>[10x]MVTTVLWGCELSQERRTWTFRPQLEGKQSCR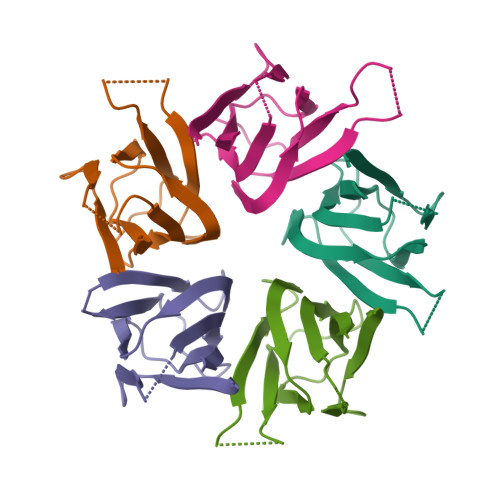LLLHTICLGEKAKEEMHRVEILPPANQEDKKMQPVTIASLQASVLPMVSMVGVQLSPPVTFQLRAGSGPVFLSGQERYE>MGKYQVMKRASEVDLSTVKYKAETMKAPHLTGLSFKLFVNLLEAPLIGSLIVDYLKKDNGMTKIFRNTVIPEEPMFRPEFPSQEPEHDVVIVGEDESPIDRLETALKCLPQYDPSRSLHADPVSSFRYWKIRDYAYAYRSKLTTPLQVAKRIISIIEEFGYDKPPTPFLIRFDANEVIKQAEASTRRFEQGNPISVLDGIFVTIKDDIDCLPHPTNGGTTWLHEDRSVEKDSAVVSKLRSCGAILLGKANMHELGMGTTGNNSNYGTTRNPHDPKRYTGGSSSGSAAIVAAGLCSAALGTDGGGSVRIPSALCGITGLKTTYGRTDMTGSLCEGGTVEIIGPLASSLEDAFLVYAAILGSSSADRYNLKPSPPCFPKLLSHNGSNAIGSLRLGKYTKWFNDVSSSDISDKCEDILKLLSNNHGCKVVEIVVPELEEMRAAHVISIGSPTLSSLTPYCEAGKNSKLSYDTRTSFAIFRSFSASDYIAAQCLRRRLMEYHLNIFKDVDVIVTPTTGMTAP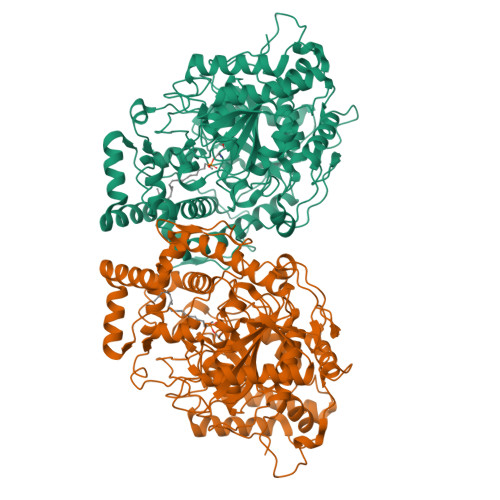VIPPDALKNGETNIQVTTDLMRFVLAANLLGFPAISVPVGYDKEGLPIGLQIMGRPWAEATVLGLAAAVEELAPVTKKPAIFYDILNTNKGEFEAYVEQKLISEEDLNSAVDHHHHHH[12x]> MEIEIKLRLPSPSAHQLLSDALSP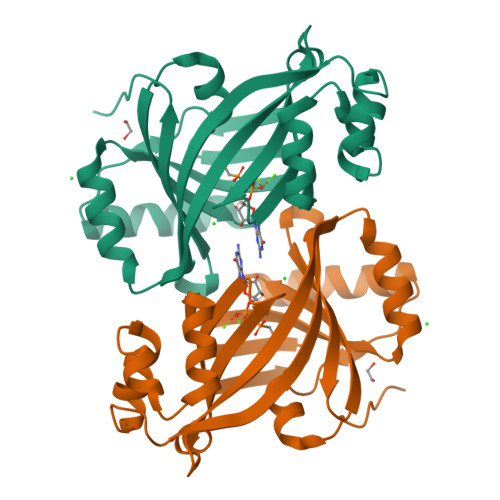FHLKTHLQHNLFFDTAAGDLASVFSALRIRFYDANAKCVLSLKSRPKLSEGVSHVEEDEEEIDPQIGQEVTANPSKMGSLLEKSRIWRRVVDEIGVADDGGEFVCLGGFRNVRAVYRWVEGLILELDETEYGFGTSYEIECETTEPERVKGLLEGFLKEKGIPYEYSGASKFAVFRSGKLLPLEHHHHHH> MKKIILGLSVLCLLMACGSSEQPAVIKVSEETLMYEVRATPSPADGTYVKVNPPRFMWPDKFPHLGPVLDGVPGQVDEKPKVVYRIRISQDKNFRKDVLTGERAWAFFN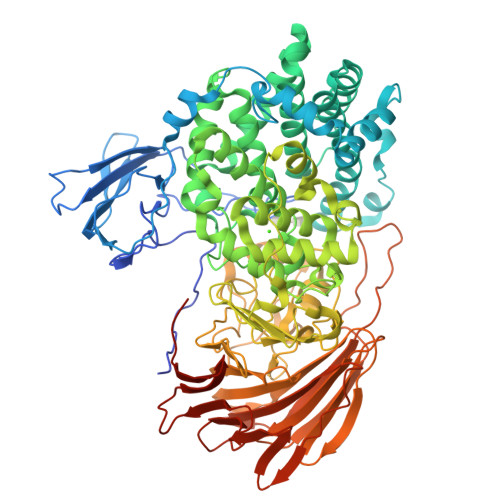PFQCLAQGKWYWQHAYVTPEGTEEWSPVYQFYIDKDTPEFNPPTLEKVLARYPSHHPRVLLDADDWENIIAKNNNNPEARTYMDKASQCISRPLKHLQEEIDTTNVVTLTNIVQRESALIRESRKIVDREEANVEALVRAYLLTKDEKYYREGINRLSEILSWQKSKYFAGDFNLSTLLSMSTSAYDGFYNLLSPEEKQLLLDNIRKIGDKFYNEYVNHLENRIADNHVWQMTFRILTMAAFATVGEIPEASVWTDYCYNEWISRLPGLHKDGGWHNGDAYFHVNIRTLIEVPVFFSRISGFNFFADPWYNNNALYVIYQQPPFSKSGGHGNSHEGQRSPNGGRIGYADALARECNNPWAAAYVHEIMQEDPDILSKAFEAKPADLTWYRCTTPKERPAYSKHLSELPESKVFKQTGTALMNTDIGHHANNAMLSFRSSPYGSTSHALANQNAFNTFFGGKAIFYSSGHRTGFTDDHCMYAYRNTRAHNSILVNGMGQKIGTEGYGWIPRYYEGEEISYVVGDASNAYGKVVSPLWLERGRLSGTQFTPEKGWDENKLEFFRRHVVQLGRSGLFVVYDELAGKEPVEWNYLLHTVELPMEVVKEEGGLRILGKNKADGISIAHLYSSQEMTYAQTDTFFVAALDWKKRLGKALPNHYHFTATTAPCNKVFFLNIIDVHGNNRADAVINHQGNHITVEGWVIECNLDSEGKAFLHIENKQNGASLDFNYNSNKGATTIVDQVDGKRIEKRLVDSLPEPEILEHHHHHH>SVTVKRIIDNTVIVPKLPANEDPVEYPADYFRKSKEIPLYINTTKSLSDLRGYVYQGLKSGNVSIIHVNSYLYGALKDIRGKLDKDWSSFGINIGKAGDTIGIFDLVSLKALDGVLPDGVSDASRTSADDKWLPLYLLGLYRVGRTQMPEYRKKLMDGLTNQCKMINEQFEPLVPEGRDIFDVWGNDSNYTKIVAAVDMFFHMFKKHECASFRYGTIVSRFKDCAALATFGHLCKITGMSTEDVTTWILNREVADEMVQMMLPGQEIDKADSYMPYLIDFGLSSKSPYWSVKNPAFHFWGQLTALLLRSTRARNARQ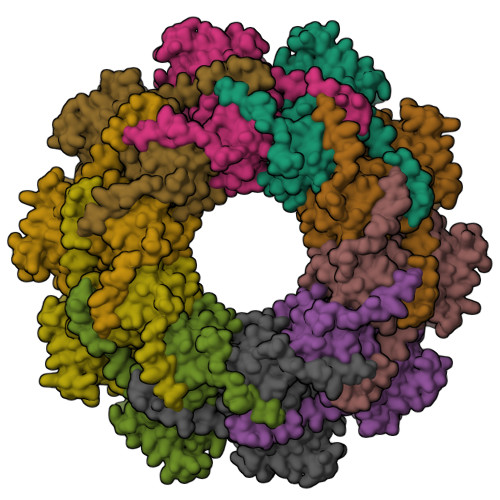PDDIEYTSLTTAGLLYAYAVGSSADLAQQFCVGDNKYTPDDSTGGLTTNAPPQGRDVVEWLGWFEDQNRKPTPDMMQYAKRAVMSLQGLREKTIGKYAKSEFDK[5x]> GSHMTAYTAERQPERDITPVNDETMQEINTLLIALDKTWDDDLLPLCSQIFRRDIRASSE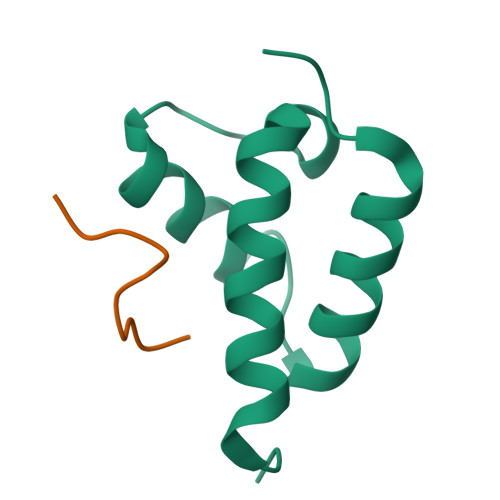LTQAEAVKALGFLKQKAAEQKVAA;> WMDFDDDIPF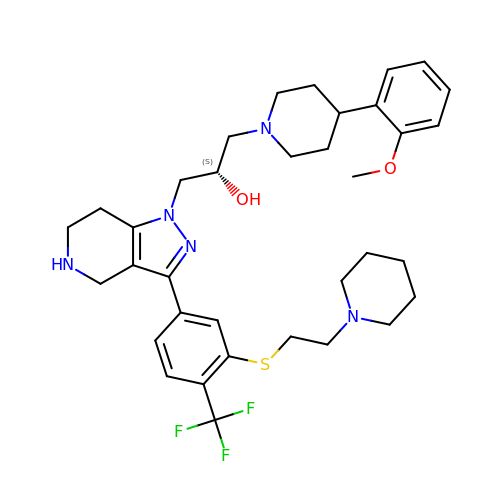(2S)-1-[4-(2-methoxyphenyl)piperidin-1-yl]-3-{3-[3-{[2-(piperidin-1-yl)ethyl]sulfanyl}-4-(trifluoromethyl)phenyl]-4,5,6,7-tetrahydro-1H-pyrazolo[4,3-c]pyridin-1-yl}propan-2-ol | C35 H46 F3 N5 O2 S | VEQXQVUVDISNGH-MHZLTWQESA-N>GSHMKITYPLPPNLPEQLPLLTNCQLEDEAILENHLYQQIDLPNQEVRNLVFRDAVFDHLSLANGQFASFDCSNVRFEACDFSNVEWLSGSFHRVTFLRCNLTGTNFADSYLKDCLFEDCKADYASFRFANFNLVHFNQT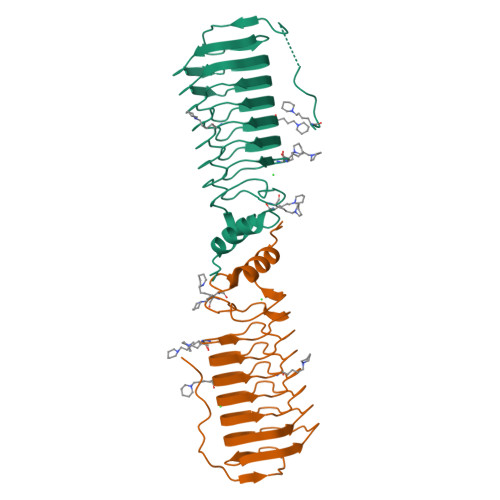RLVESEFFEVTWKKLLLEACDLTESNWLNTSLKGLDFSQNTFERLTFSPNYLSGLKVTPEQAIYLASALGLVIT[2x]> MRLCRRLSYHAYVPKGASVQMGETFMPSNIATAVFRETEAAAARADKTKEETGFFSQPRLNYPVSSGIPALFSKDQFDMQYSLFHRDVVETLNRHTLGTPLEGHNLETVIRKTSFDATQAVAHTAASEHFNYCFFYKSLRPWGTAPPPRLRE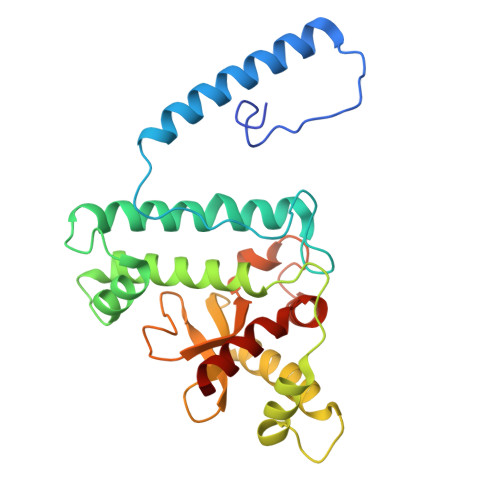ALQLQYGTNGSADAMDEVRRIVWVTAASHQERCGWVYLVWSGVHFDVVEFPHGSCPIASDLIPLLALNVHESAYILDYGTSGLKQYVENYFKACNWPLAERYYLMAIGQVV> MQEIKRINKIRRRLVKDSNTKKAGKTGPMKTLLVRVMTPDLRERLENLRKKPENIPQPISNTSRANLNKLLTDYTEMKKAILHVYWEEFQKDPVGLMSRVAQPAPKNIDQRKLIPVKDGNERLTSSGFACSQCCQPLYVYKLEQVNDKGKPHTNYFGRCNVSEHERLILLSPHKPEANDELVTYSLGKFGQRALDFYSIHVTRESNHPVKPLEQIGGNSCASGPVGKALSDACMGAVASFLTKYQDIILEHQKVIKKNEKRLANLKDIASANGLAFPKITLPPQPHTKEGIEAYNNVVAQIVIWVNLNLWQKLKIGRDEAKPLQRLKGFPSFPLVERQANEVDWWDMVCNVKKLINEKKEDGKVFWQNLAGYKRQEALLPYLSSEEDRKKGKKFARYQFGDLLLHLEKKHGEDWGKVYDEAWERIDKKVEGLSKHIKLEEERRSEDAQSKAALTDWLRAKASFVIEGLKEADKDEFCRCELKLQKWYGDLRGKPFAIEAENSILDISGFSKQYNCAFIWQKDGVKKLNLYLIINYF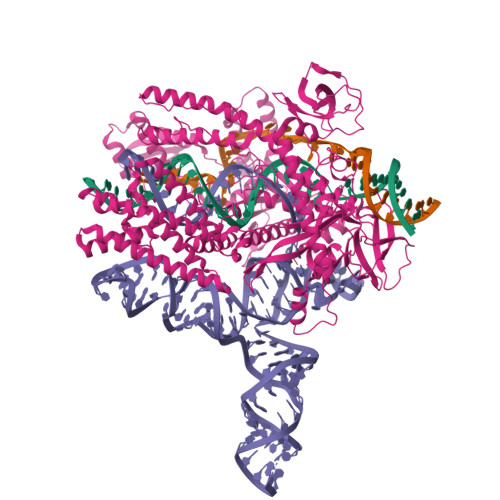KGGKLRFKKIKPEAFEANRFYTVINKKSGEIVPMEVNFNFDDPNLIILPLAFGKRQGREFIWNDLLSLETGSLKLANGRVIEKTLYNRRTRQDEPALFVALTFERREVLDSSNIKPMNLIGIARGENIPAVIALTDPEGCPLSRFKDSLGNPTHILRIGESYKEKQRTIQAAKEVEQRRAGGYSRKYASKAKNLADDMVRNTARDLLYYAVTQDAMLIFANLSRGFGRQGKRTFMAERQYTRMEDWLTAKLAYEGLPSKTYLSKTLAQYTSKTCSNCGFTITSADYDRVLEKLKKTATGWMTTINGKELKVEGQITYYNRYKRQNVVKDLSVELDRLSEESVNNDISSWTKGRSGEALSLLKKRFSHRPVQEKFVCLNCGFETHAAEQAALNIARSWLFLRSQEYKKYQTNKTTGNTDKRAFVETWQSFYRKKLKEVWKPAV>SSGLVPRGPLGSHMDAVDATMEKLRAQCLSRGASGIQGLARFFRQLDRDGSRSLDADEFRQGLAKLGLVLDQAEAEGVCRKWDRNGSGTLDLEEFLRALRPPMSQAREAVIAAAFAKLDRSGDGVVTVDDLRGVYSGRAHPKVRSGEWTEDEVLRRFLDNFDSSEKDGQV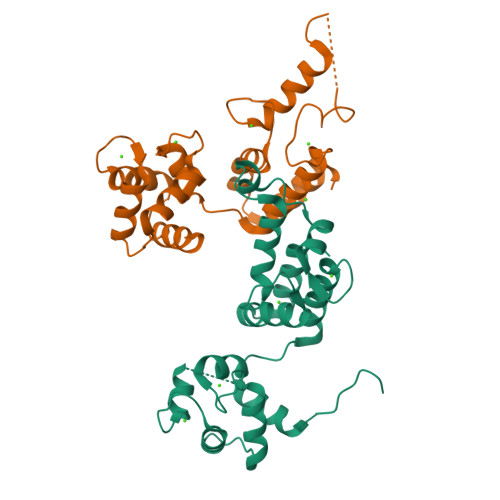TLAEFQDYYSGVSASMNTDEEFVAMMTSAWQLKL[2x]>[2x]CG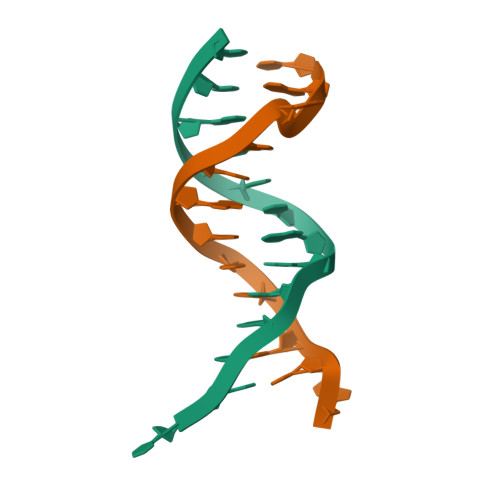CAGAATTCGCG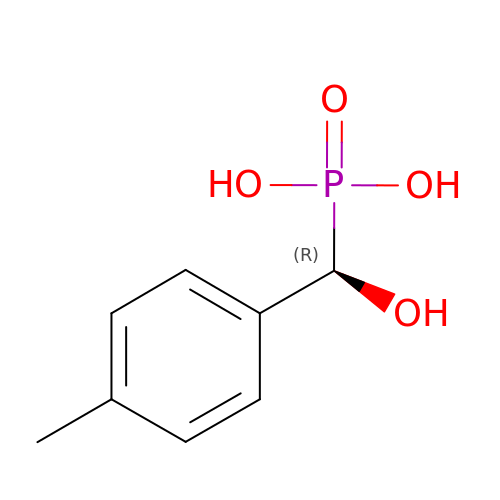[(R)-hydroxy(4-methylphenyl)methyl]phosphonic acid | C8 H11 O4 P | AFOAUCXHAIELNA-MRVPVSSYSA-N>[4x]GIDPFTMKYVGSIDQGTTSTRFIIFDERQRPVSVHQVPHTQHTPHPGWLEHDPMEIFRSACKCMSVAIAKLRQKDASFRKIEAIGITNQRETTVAWDRVTKEPLCYAPVWNDLRTYDITKKVTAELGGGDSMFASKITGLPVSTYFAAFKMRWMLENVPAVADACRRGTLCFGTIDTWLMYKLSGGKAFVTDVTNASRTFLMDLRTR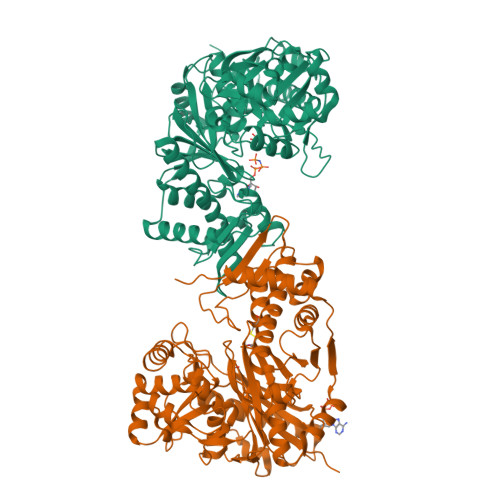KWSPELCEKLKIPMETLPEIRSNSELFGYVETDECGVAAALNERTPIMGSIGDQQSALFGNMCFEKGEAKNTYGTGCFLLMNVGEEARFSKHGLLSTVGFQVGRDGPCYYALEGAIACAGATVEWMRRNMNLFSHITECEKLARSVPGTQGIVFVPAFSGLLAPYWDPSARGTIVGMTLKTTRAHVIRAALQAIALQLNDVVGSMKRDAGLNLSSLRVDGGLSKNGLLMEIQASLLGVDILVPSMHETTALGAALCAGLAAGVWTSLEEVKAVSRRENSWKTVSPSGSAMEREAMIAEWREALKRTKWAKL(1R,2R,3R,4S,5R)-4-(BENZYLAMINO)-5-(METHYLTHIO)CYCLOPENTANE-1,2,3-TRIOL | C13 H19 N O3 S | 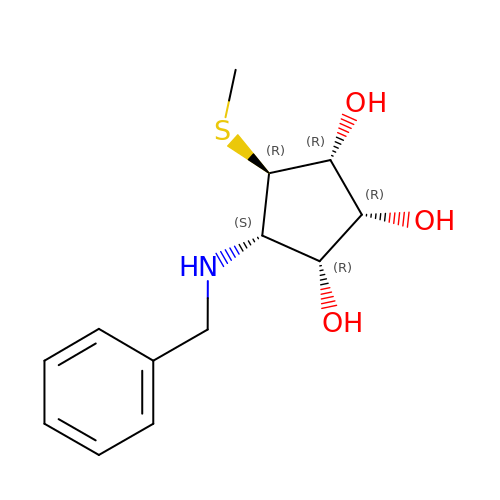CHTYSDQNKZIWBZ-ZOLYEBIHSA-N>MEVYYTSLRCRCVQESSVFIPRRFIDRIQILPRGNGCPRKEIIVWKKNKSIVCVDPQAEWIQRMMEVLRKRSSSTLPVPVFKRKIP[7x]

CXCL13 is the cognate chemokine agonist of CXCR5, a class A G-protein-coupled receptor (GPCR) that is essential for proper humoral immune responses. CXCL13 is an agonist of CXCR5, activating the receptor, resulting in downstream calcium signaling and ultimately the chemotactic response for which chemokines are named. As elucidated from structural data on many chemokines, this conserved tertiary structure consists of a disordered N-terminal region (6–10 amino acids, referred to here as the chemokine N-terminus), followed by a long loop known as the ‘N-loop’ ending in a short 310-helix, a three-stranded β-sheet and a C-terminal α-helix. Furthermore, we were able to utilize two of these mutants to solve the first uncomplexed crystal structures of human CXCL13. These structures allowed us to observe that the core domain of CXCL13 (i.e. everything except its N- and C-termini) is fairly rigid, whereas its N-terminus exhibits striking flexibility as well as a propensity to form both intramolecular and intermolecular β-strand interactions.

We found that both V1M and Δ1L2M CXCL13 functioned as agonists, with EC50 values of 5.64 and 133 nM, respectively. In terms of efficacy, V1M CXCL13 was the most efficacious construct other than WT CXCL13, attaining 93.6% activity at 1 µM, whereas Δ1L2M CXCL13 was only able to achieve a mere 55.1% activity at the same concentration. The loss of contacts at residue 1 are a likely culprit for the significantly decreased efficacy of this construct, suggesting that residue 1 plays a critical role in triggering the activation of CXCR5. We were also very intrigued to note that once again the N-terminus of Δ1L2M CXCL13 formed additional β-strand interactions, although they were different from those seen in the Met CXCL13 structure. Specifically, we observed that the N-terminus of each monomer exhibits an extreme turn away from its core domain and then folds into a β-strand (β−1) which interacts in an antiparallel fashion with both the three-stranded core β-sheet from an adjacent monomer as well as an induced β-strand formed by the N-loop within the same monomer (β0). By aligning the seven monomers found within the asymmetric unit of the Δ1L2M CXCL13 structure, we were able to observe that they are all extremely similar prior to their C-terminal ends, with only minor fluctuations found in their N-termini and in the β1–β2 loop region. All monomers exhibited density beginning at the N-terminal residue Met2, with the exception of one chain that began at Glu3. The final C-terminal residue varied between monomers, with the shortest monomer ending at Arg72 and the longest monomer ending at Lys83. The alignments also showed that the largest observable differences between the monomers was in their C-terminal regions following the α1 helix, also known as the C-terminal extension.> VPRGSHMKKLLVANRGEIAVRVFRACNELGLSTVAVYAREDEYSVHRFKADESYLIGQGKKPIDAYLDIDDIIRVALESGADAIHPGYGLLSENLEFATKVRAAGLVFVGPELHHLDIFGDKIKAKAAADEAKVPGIPGTNGAVDIDGALEFAKTYGYPVMIKAALGGGGRGMRVARNDAEMHDGYARAKSEAIGAFGSGEIYVEKYIENPKHIEVQILGDRHGNIIHLHERDCSVQRRNQKVIEIAPAVGLSPDFRNEICEAAVKLCKNVGYVNAGTVEFLVKDDKFYFIEVNPRVQVEHTITELITGVDIVQAQILIAQGKDLHREIGLPAQSEIPLLGSAIQCRITTEDPQNGFLPDTGKIDTYRSPGGFGIRLDVGNAYAGYEVTPYFDSLLVKVCTFANEFSDSVRKMDRVLHEFRIRGVKTNIPFLINVIANENFTSGQATTTFIDNTPSLFNFPRLRDRGTKTLHYLSMITVNGFPGIENTEKRHFEEPRQPLLNLEKKKTAKNILDEQGADAVVDYVKNTKEVLLTDTTLRDAHQSLLATRLRLQDMKGIAQAIDQGLPELFSAEMWGGATFDVAYRFLNESPWYRLRKLRKLMPNTMFQMLFRGSNAVGYQNYPDNVIEEFIRVAAHEGIDVFRIFDSLNWLPQMEKSIQAVRDNGKIAEATICYTGDILDPSRPKYNIQYYKDLAKELEATGAHILAVKDMAGLLKPQAAYRLISELKDTVDLPIHLHTHDTSGNGIITYSGATQAGVDIIDVATASLAGGTSQPSMQSIYYALEHGPRHASINVKNAEQIDHYWEDVRKYYAPFEAGITSPQTEVYMHEMPGGQYTNLKSQAAAVGLGHRFDEIKQMYRKVNMMFGDIIKVTPSSKVVGDMALFMIQNDLTEEDVYARGNELNFPESVVSFFRGDLGQPVGGFPEKLQKIIVKDKAVITDRPGLHAEKVDFETVKADLEQKIGYEPGDHEVISYIMYPQVFLDYQKMQREFGAVTLLDTPTFLHGMRLNEKIEVQIEKGKTLSIRLDEIGEPDLAGNRVLFFNLNGQRREVVINDQSVQAQVVAKRKAETGNPNQIGATMPGSVLEILVKAGDKVQKGQALMVTEAMKMETTIEAPFDGEIVDLHVVKGEAIQTQDLLIEIN

Pyruvate carboxylase (PC) is a tetrameric enzyme that contains two active sites per subunit that catalyze two consecutive reactions. A mobile domain with an attached prosthetic biotin links both reactions, an initial biotin carboxylation and the subsequent carboxyl transfer to pyruvate substrate to produce oxaloacetate. PC is mostly found as tetramers of four identical subunits, with monomers of ~120–130 kDa in size. This enzyme possesses a tetrahedral geometry with the tetramer organized in two layers. In this work, we study the structure of Lactococcus lactis PC (LlPC) during catalysis in the presence of positive allosteric regulator acetyl-CoA.

A focused classification with a mask around the CT domain produced: a class with no substrate CTempty; two classes with pyruvate CTpyr; a class with BCCP inserted at the active site CTreact; and five classes with oxaloacetate CToxa. The cryoEM maps of these catalytic states show local densities that define the nature of the bound molecules with high definition, and also large differences in the degree of openness of the CT domain, being very open in the CTempty class, intermediate at variable degrees within CTpyr and CToxa classes, and highly closed in the CTreact class with bound BCCP domain (left panels in Fig. 5 and Supplementary Movie M2). During the transition from CTempty to CTpyr or CToxa, the 825–935 region, a subdomain of the funnel, closes and moves closer to the active site. The loop 608–618 of the TIM barrel also moves with the funnel. The main catalytic residues of the CT domain are placed in a TIM barrel (residues 525-780). This region is very well-resolved in the volumes, allowing the identification of most of the side chains, ligands and even some water molecules.>[6x]EEGQKVDHCARHGEKLLLFCQEDSKVICWLCERSQEHRGHHTFLMEEVAQEYHVKLQTALEMLRQKQQEAETERNQVAKRVPKAPPEEKEALIARGKALGEQTQYMRELISELEHRLQGSMMDLLQGVDGIIKRIENMTLK

TRIM5α is a restriction factor that intercepts the incoming capsids of diverse retroviruses, including HIV-1, and inhibits viral replication. Like all TRIM proteins, TRIM5α consists of an N-terminal tripartite or RBCC motif (RING, B-box 2, and coiled-coil domains), followed by a C-terminal domain. Higher-order assembly of TRIM5α requires the B-box 2 domain, which is thought to mediate three-fold symmetric interactions that connect coiled-coil mediated TRIM5α dimers into a hexagonal net. We therefore engineered artificial constructs – which we call miniTRIMs – that retain the integrated B-box/coiled-coil fold of the full-length dimer but are more amenable to biochemical and structural analyses.

A P212121 crystal contained two trimers in the asymmetric unit (3.26 Å resolution, R/Rfree = 0.26/0.30), a C2 form contained one dimer (2.1 Å, R/Rfree = 0.18/0.22), and a P1 form contained two dimers (2.3 Å, R/Rfree = 0.22/0.26). The Bcc miniTRIM trimer is organized as a triskelion: three B-box 2 domains make a central three-fold symmetric vertex from which the coiled-coil domains emanate as spokes. As expected, the trimerization interactions are principally mediated by the B-box domain, burying 578 Å2 of the available surface area from each subunit. The B-box packs against the N-terminal end of the coiled-coil helix through a hydrophobic interface (asterisks), suggesting that trimer formation requires the presence of the coiled-coil. The Trp117 indoles in the trimer form a channel that would be expected to have a highly negatively charged hole at the center, which is likely to be partially stabilized by the positively charged Arg121 sidechains. Comparison of the trimer and dimer bonding interactions revealed that the two oligomers are distinguished primarily by intermolecular packing between the Trp117, Leu118, and Leu132 sidechains in the hydrophobic layer. In particular, Leu118 and Leu132, which are located at the outer edges of the binding surface, are in van der Waals contact in the trimer, but more separated in the dimer. In context of the trimer, the three coiled-coils do not contact each other and can therefore move independently. Nevertheless, it seems clear that the B-box trimer is what facilitates hexagonal lattice assembly, at least in vitro.>MTAVEFIEPLTHEEGVSQATKLFVDTYGAAPEGVWAAPGRVNLIGEHTDYNAGLCLPIALPHRTFIALKPREDTKVRVVSGVAPDKVAEADLDGLKARGVDGWSAYPTGVAWALRQAGFDKVKGFDAAFVSCVPLGSGLSSSAAMTCSTALALDDVYGLGYGDSDAGRVTLINAAIKSENEMAGASTGGLDQNASMRCTEGHALLLDCRPELTPLENVSQQEFDLDKYNLELLVVDTQAPHQLNDGQYAQRRATCEEAAKILGVANLRVTADGISKADDQFQALKETLDALPDETMKKRVRHVVTEIERVRSFVRAFAQGDIKAAGRLFNASHDSLAADYEVTVPELDIAVDVARKNGAYGARMTGGGFGGSIIALVDKGQGHEIAQKIADRFEKEGFNAPRALPAF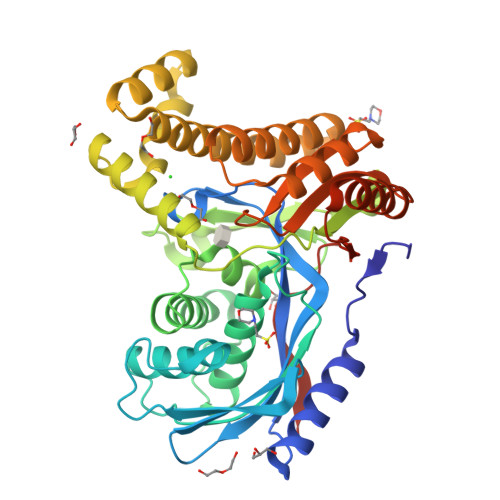AAASASREAKLAAALEHHHHHH[4x]>[3x]SNAEKWTSTAIITQPDVGQIAGYNNAMNVIYGQAAPKVSDLQETLIGRFSSAFSALAETLDNQEEPE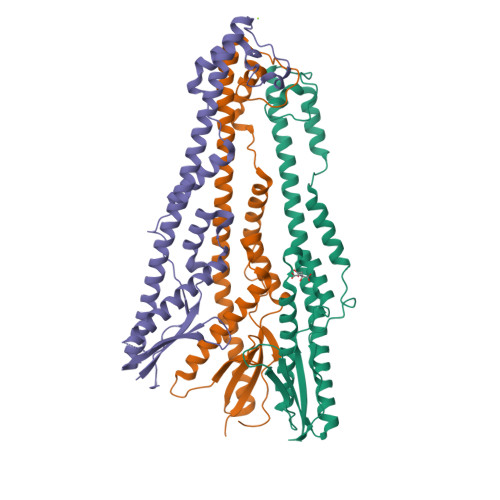KLTIEPSVKNQQLPLTVSYVGQTAEGAQMKLAQYIQQVDDKVNQELEKDLKDNIALGRKNLQDSLRTQEVVAQEQKDLRIRQIQEALQYANQAQVTKPQVQQTEDVTQDTLFLLGSEALESMIKHEATRPLVFSPNYYQTRQNLLDIEKLKFDDLDIHAYRYVMKPTLPIRRDSPK{2-[(2R,3R,4R,5R)-3-(alpha-D-glucopyranosyloxy)-4-hydroxy-2,5-bis(hydroxymethyl)pyrrolidin-1-yl]ethyl}phosphonic acid | C14 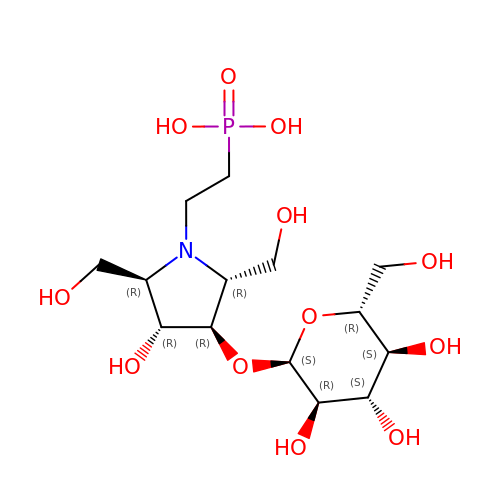H28 N O12 P | QLKUMDMMFYIFJS-IDWYSJKESA-N>XGEIAQSIKEIA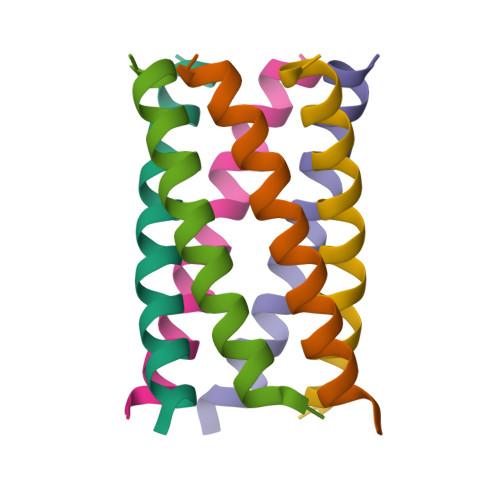KSIKEIAWSIKEIAQSIKG[4x]> MDAELKIFVSSQHQPDIWRKALDQYEAKTPGVKVVIETGGNTSEMQAQYLNTVMSAKDSSLDVLMLDVIRPAQFATAGWTSDFSGKDLSAYLPTYAEANTVNGKIVALPAFADSMF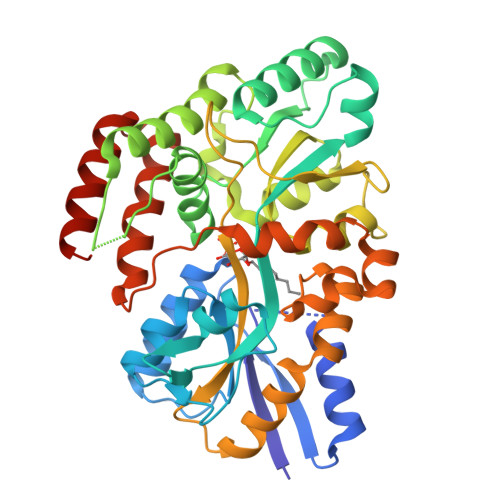LYYRKDLLDKYGIKPPTTWDELKEASKKVMEGEKNPELQGLSFQGKAIEGAVCTFLLPYWSEGKSLVENGKLNFDNKAAVDSLKLWKSFVDDGISKKNISEVATDDTRKEFQAGKVLFAVNWSYAWTHFQGKESQVNDKVGVARLPAVKGGEQTTCLGGWEFGVSAYSKQQDEAKKLVEYLSSQDVSKFMAINAALLPTYAALYKDADVTKTIPWFADALPVVETAKARPVTPRYNEVSETIRTTVNGVLAGVMTPEDGAKQMESRLRRVLRLEHHHHHH> MSNETLSADVVIIGAGICGSLLAHKLVRNGLSVLLLDAGPRRDRSQIVENWRNMPPDNKSQYDYATPYPSVPWAPHTNYFPDNNYLIVKGPDRTAYKQGIIKGVGGTTWHWAASSWRYLPNDFKLHSTYGVGRDYAMSYDELEPYYYEAECEMGVMGPNGEEITPSAPRQNPWPMTSMPYGYGDRTFTEIVSKLGFSNTPVPQARNSRPYDGRPQCCGNNNCMPICPIGAMYNGVYAAIKAEKLGAKIIPNAVVYAMETDAKNRITAISFYDPDKQSHRVVAKTFVIAANGIETPKLLLLAANDRNPHGIANSSDLVGRNMMDHPGIGMSFQSAEPIWAGGGSVQMSSITNFRDGDFRSEYAATQIGYNNTAQNSRAGMKALSMGLVGKKLDEEIRRRTAH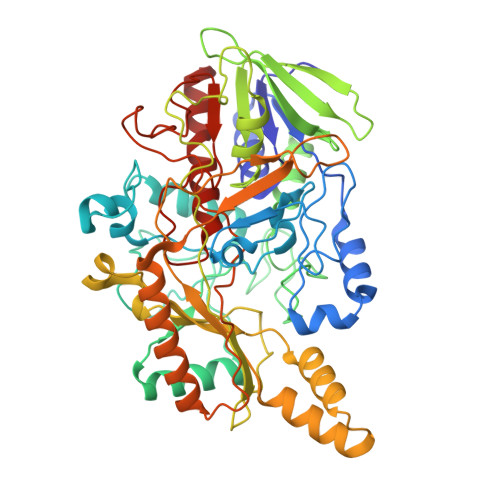GVDIYANHEVLPDPNNRLVLSKDYKDALGIPHPEVTYDVGEYVRKSAAISRQRLMDIAKAMGGTEIEMTPYFTPNNHITGGTIMGHDPRDSVVDKWLRTHDHSNLFLATGATMAASGTVNSTLTMAALSLRAADAILNDLKQG> HPICEVSKVASHLEVNCDKRQLTAL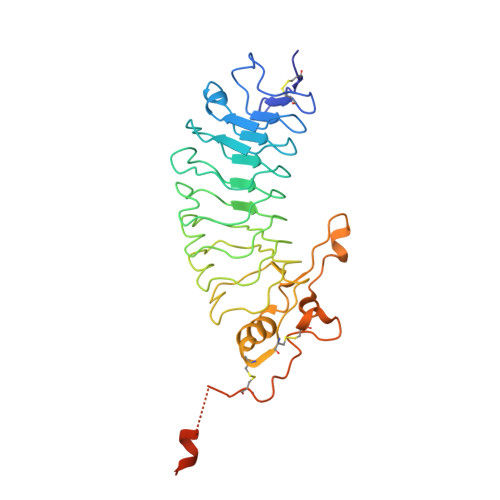PPDLPKDTTILHLSENLLYTFSLATLMPYTRLTQLNLDRCELTKLQVDGTLPVLGTLDLSHNQLQSLPLLGQTLPALTVLDVSFNRLTSLPLGALRGLGELQELYLKGNELKTLPPGLLTPTPKLEKLSLANNQLTELPAGLLNGLENLDTLLLQENSLYTIPKGFFGSHLLPFAFLHGNPWLCNCEILYFRRWLQDNAENVYVWKQGVDVKAMTSNVASVQCDNSDKFPVYKYPGKGCPTLGDEGDTDLYDYYPEEDTEGDKVRATRTVVKFPTKAHTT> PDMFCALKIKFFLEIGDEDAARKAAKKCG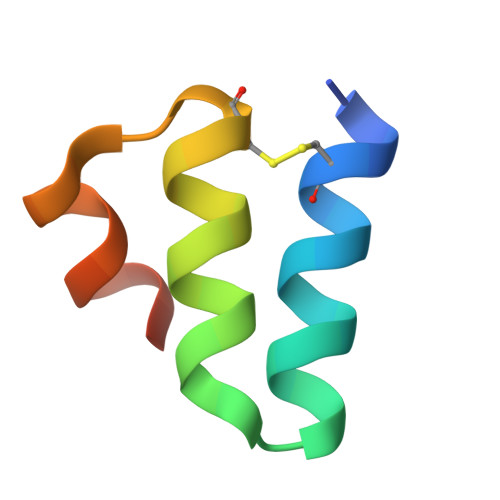YSEEQAERIIKKNL> MKVISLKKDSFNKGGAVITLLPEDKEDLFTVYQIVDKDDELIFKKKFTSKLDEAGKKKSTDLVKLKIKVISEDFDMKDEYLKYKGVTVTDESGASNVDIPVGKYLSFTLDYVYPFTIIKQNFNKFMQKLLNEACNIEYKSDTAAVVLQEGIAHVCLVTSSSTILKQKIEYSMPKKKRTTDVLKFDEKTEKFYKAIYSAMKKDLNFDKLKTIILCSPGFYAKILMDKIFQYAEEEHNKKILDNKGMFFIAHCSTGYLQGINEVLKNPLYASKLQDTKYSKEIMVMDEFLLHLNKDDDKAWYGEKEVVK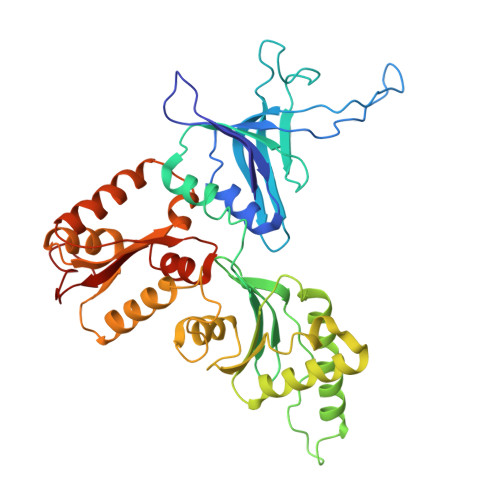AAEYGAISYLLLTDKVLHSDNIAQREEYLKLMDSVESNGGKALVLSTLHSLGEELDQLTGIACILKYPLPDLDEDDGEE> MKHHHHHHHGAAGTSLYKKAGENLYFQGSMESLFPNKGEIIRELLKDPLILKNDSKRSNGSELELDSSDLLQREAILANELNILDNLKTFLNLIKEVKTNLNILELENCYYSLQSLRKKMRNNAAYLKQSFNFQQSISTYVDTLHLELVSTLYKILTNGFWKITENSIQFTPTVEWGKDKVHIEYDTFMDFVAQQYFPKGSLDNQAWFILDMTSADSQEQVRAKLNTIMKEYMNLSRIVSMIKNSIFISGKEISYENEKNILVFSKSSSHGQHCVSTVLTSFEAVCDFMLDGLAFRDRKTLSYELGPLFNTEFTKFVKNNASII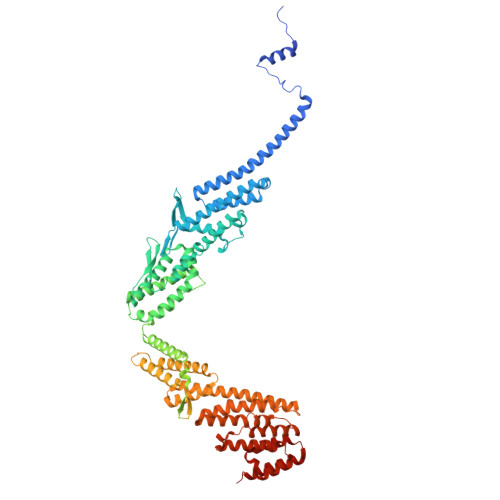LESLDSPLKNLVSVINNKLTRLVAKSEVTNWTHSGKEIQDLLMNKQLYYNLLLDKVLESHISEIRSIFEDPKKSWQNLEVVELTTSNTNTMSEKIGKNDSDVQNEKELHNAVSKDDDWNWEVEDDDADAWGDEIDVNIDDEEEKTNQEKEKEPEEEENAWDEAWAIDENIDDASLENGKEHLKAHDVGSLDKDHIEVTQLPKLFLAISQNFKSSFADSHVDEQYFAYKYNLLQTSYMAMCTANFSHNWCQLYVDMRYLIERDEKLYRIKELTRNLLETKLNMKYRIVCQLIRHQLTEFRENERNPSWDATIEKLLPYILKEIVRPLQKIRGEEGSRYLLSFLNFLYNDCVTKEILKWQIISEVNSENLGELVSLLVNNTDIQLLAKEPSYKKMREKFATMGKFLPLHLKEIMEMFYNGDFYLFATDELIQWIELLFADTPLRRNAIDDIYEIRGTALDD> VGSNSYPHK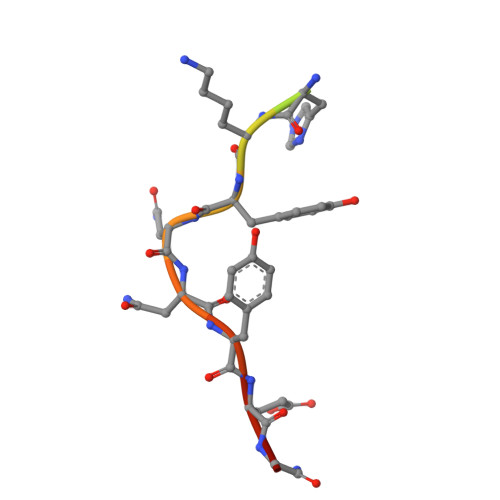YNNYEGX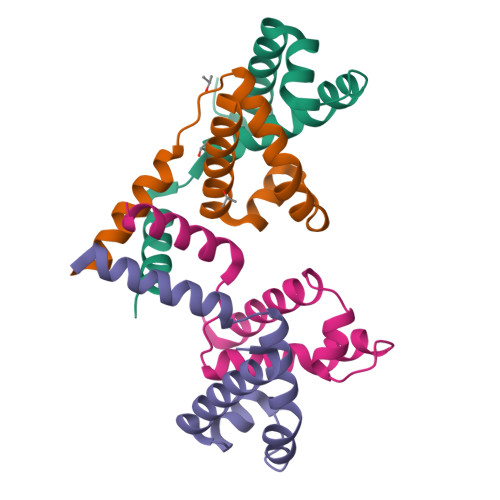>[4x]MVRANKRNEALRIESALLNKIAMLGTEKTAEAVGVDKSQISRWKRDWIPKFSMLLAVLEWGVVDDDMARLARQVAAILTNKKRPAATERSEQIQMEF> MEPGPTAAQRRCSLPPWLPLGLLLWSGLALGALPFGSSPHRVFHDLLSEQQLLEVEDLSLSLLQGGGLGPLSLPPDLPDLDPECRELLLDFANSSAELTGCLVRSARPVRLCQTCYPLFQQVVSKMDNISRAAGNTSESQSCARSLLMADRMQIVVILSEFFNTTWQEANCANCLTNNS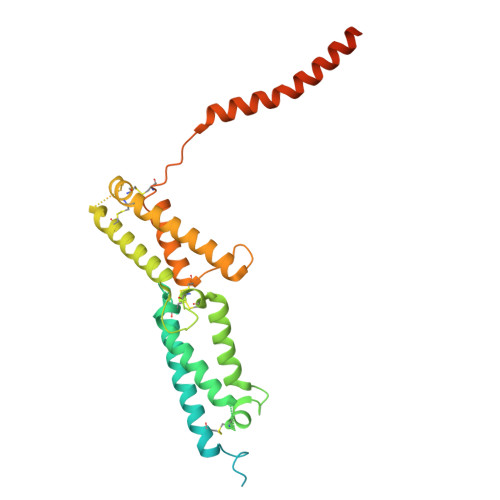EELSNSTVYFLNLFNHTLTCFEHNLQGNAHSLLQTKNYSEVCKNCREAYKTLSSLYSEMQKMNELENKAEPGTHLCIDVEDAMNITRKLWSRTFNCSVPCSDTVPVIAVSVFILFLPVVFYLSSFLHSEQKKRKLILPKRLKSSTSFANIQENSN> MAPKAKIVLVGSGMIGGVMATLIVQKNLGDVVLFDIVKNMPHGKALDTSHTNVMAYSNCKVSGSNTYDDLAGADVVIVTAGFTKAPGKSDKEWNRDDLLPLNNKIMIEIGGHIKKNCPNAFIIVVTNPVDVMVQLLHQHSGVPKNKIIGLGGVLDTSRLKYYISQKL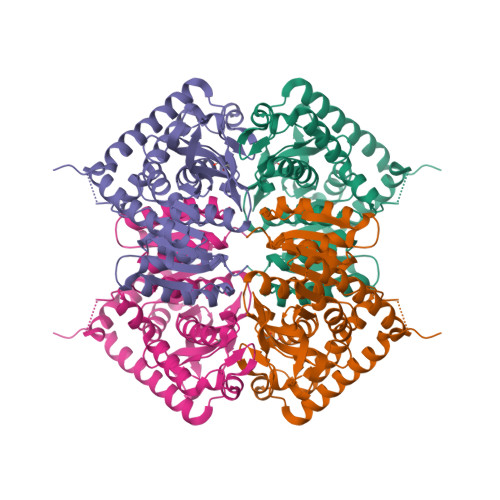NVCPRDVNAHIVGAHGNKMVLLKRYITVGGIPLQEFINNKLISDAELEAIFDRTVNTALEIVNLHASPYVAPAAAIIEMAESYLKDLKKVLICSTLLEGQYGHSDIFGGTPVVLGANGVEQVIELQLNSEEKAKFDEAIAETKRMKALAHHHHHH>MGNSGFYLYNTQNCVFADNIKVGQMTEPLKDQQIILGTTSTPVAAKMTASDGISLTVSNNPSTNASITIGLDAEKAYQLILEKLGDQILQGIADTIVDSTVQDILDKITTDPSLGLLKAFNNFPITNKIQCNGLFTPRNIETLLGGTEIGKFTVTPKSSGSMFLVSADIIASRMEGGVVLALVREGDSKPYAISYGYSSGVPNL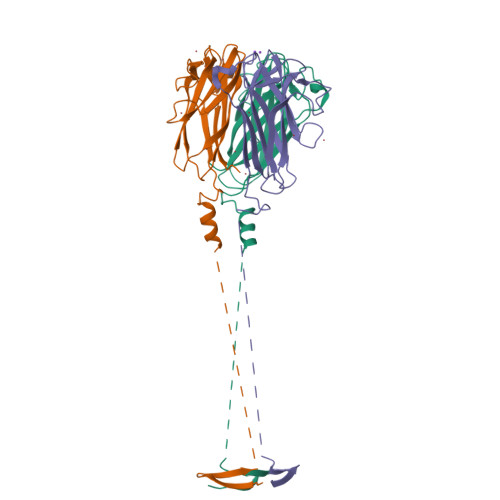CSLRTRIINTGLTPTTYSLRVGGLESGVVWVNALSNGNDILGITNTSNVSFLEVIPQTNA[6x]>[2x]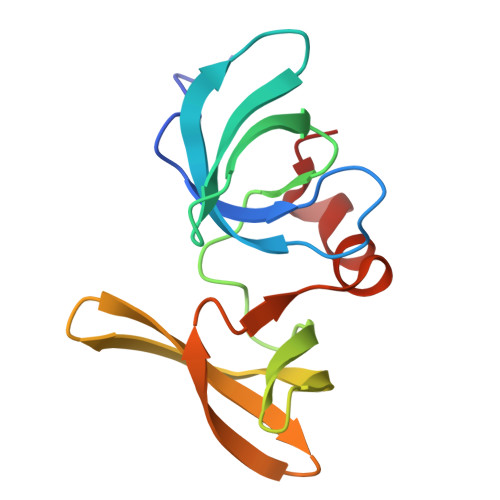GHMNSFVGLRVVAKWSSNGYFYSGKITRDVGAGKYKLLFDDGYECDVLGKDILLCDPIPLDTEVTALSPNEYFSAGVVKGHRKESGELYYSIEKEGQRKWYKRMAVILSLEQGNRLREQYGLG>MSARRTESDIQGFHATPEFGGNLQKVLVDLIELSLQGKQAHWNVVGSNFRDLHLQLDELVDFAREGSDTIAERMRALDAVPDGRSDTVAATTTLPEFPAFERSTADVVDLITTRINATVDTIRRVHDAVDAEDPSTADLLHGLIDGLEKQAWLIRSENRKV[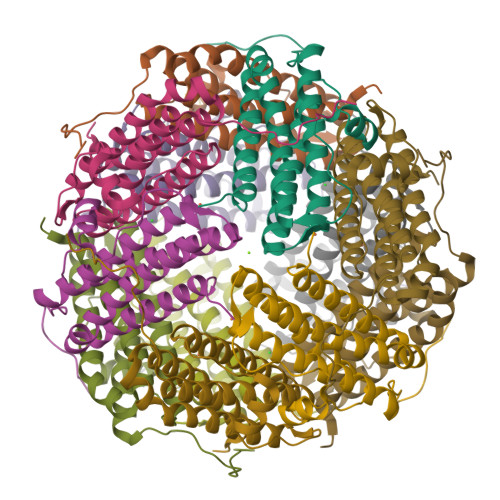4x]1H-imidazole-2-sulfonamide | C3 H5 N3 O2 S | 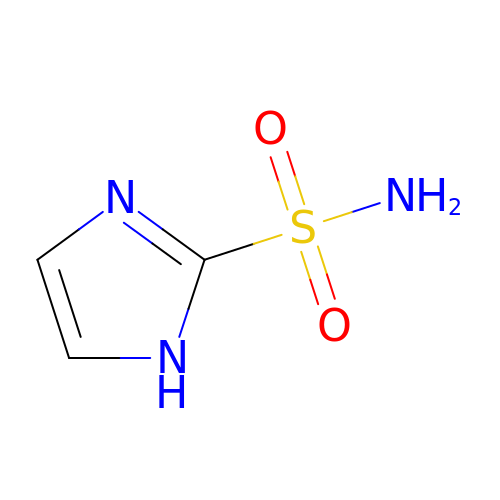PMTLRCDQMKXMRZ-UHFFFAOYSA-N>MGSSHHHHHHSSGLGVLPGGPLHMEEKLAVSLQEALQEGDTRALREVLEEIHPQDLLALWDELKGEHRYVVLTLLPKAKAAEVLSHLSPEEQAEYLKTLPPWRLREILEELSLDDLADALQAVRKEDPAYFQRLKDLLDPRTRAEVEALARYEEDEAGGLMTPEYVAVREGMTVEEVLRFLRRAAPDAETIYYIYVVDEKGRLKGVLSLRDLIVADPRTRVAEIMNPKVVYVRTDTDQEEVARLMADYDFTVLPVVDEEGRLVGIVTVDDVLDVLEAEATEDIHKLGAVDVPDLVYSEAGPVALWLARVRWLVILILTGMVTSSILQGFESVLEAVTALAFYVPVLLGTGGNTGNQSATLIIRALATRDLDLRDWRRVFLKEMGVGLLLGLTLSFLLVGKVYWDGHPLLLPVVGVSLVLIVFFANLVGAMLPFLL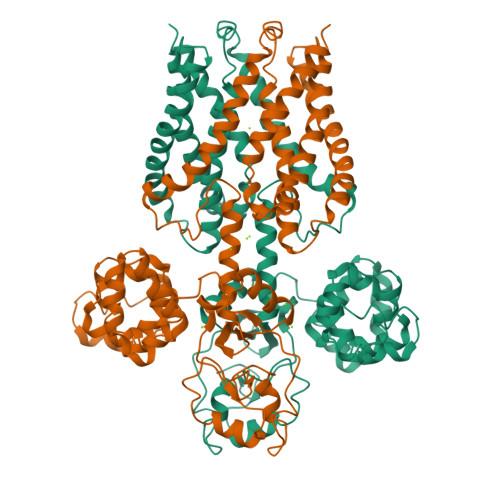RRLGVDPALVSNPLVATLSDVTGLLIYLSVARLLLEAV[4x]> MQEPLAAGAVILRRFAFNAAEQLIRDINDVASQSPFRQMVTPGGYTMSVAMTNCGHLGWTTHRQGYLYSPIDPQTNKPWPAMPQSFHNLCQRAATAAGYPDFQPDACLINRYAPGAKLSLHQDKDEPDLRAPIVSVSLGLPAIFQFGGLK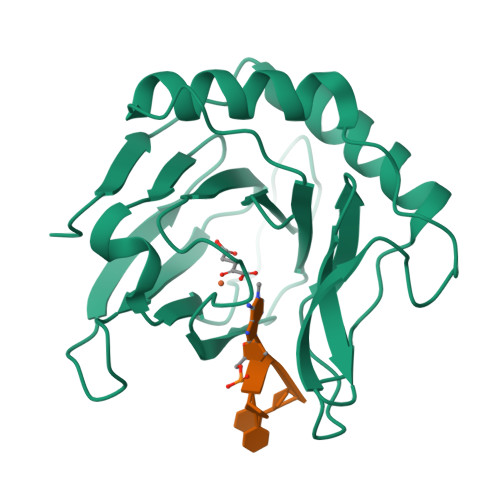RNDPLKRLLLEHGDVVVWGGESRLFYHGIQPLKAGFHPLTIDCRYNLTFRQAGKKENLYFQ>PVDVSVSIFINKIYGVNTLEQTYKVDGYIVAQWTGKPRKTPGDKPLIVENTQIERWINNGLWVPALEFINVVGSPDTGNKRLMLFPDGRVIYNARFLGSFSNDMDFRLFPFDRQQFVLELEPFSYNNQQLRFSDIQVYTENIDNEEIDEWWIRGKASTHISDIRYDHLSSVQPNQNEFSRITVRIDAVRNPSYYLWSFILPLGLIIAASWSVFWLESFSERLQTSFTLMLTVVAYAFYTSNILPRLPYTTVIDQMIIAGYGSIFAAILLIIFAHHRQANGVEDDLLIQRCRLAFPL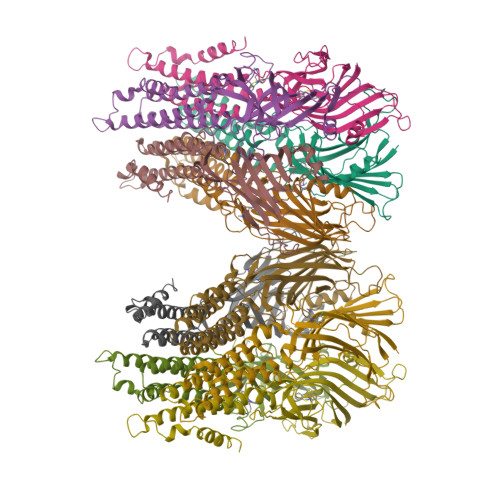GFLAIGCVLVI[10x]>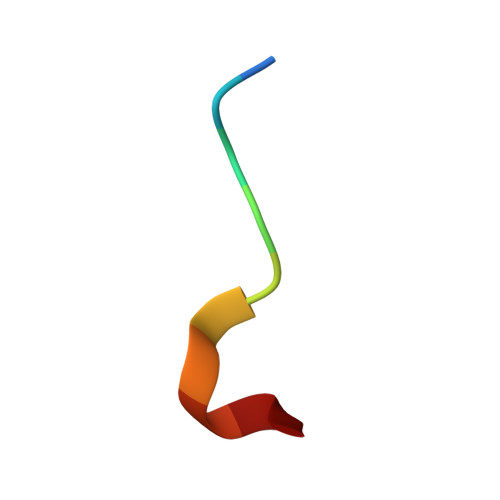 DDLDVPSFLQ(5R,6R,7R,8S)-8-(ACETYLAMINO)-6,7-DIHYDROXY-5-(HYDROXYMETHYL)-N-PHENYL-1,5,6,7,8,8A-HEXAHYDROIMIDAZO[1,2-A]PYRIDINE-2-CARBOXAMIDE 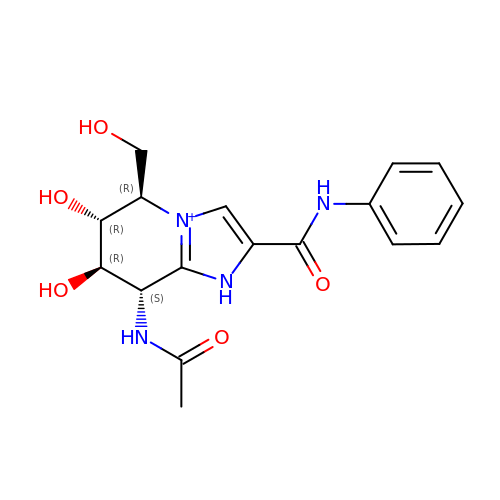| C17 H21 N4 O5 | WWSQBPPKQTUEDT-KBUPBQIOSA-O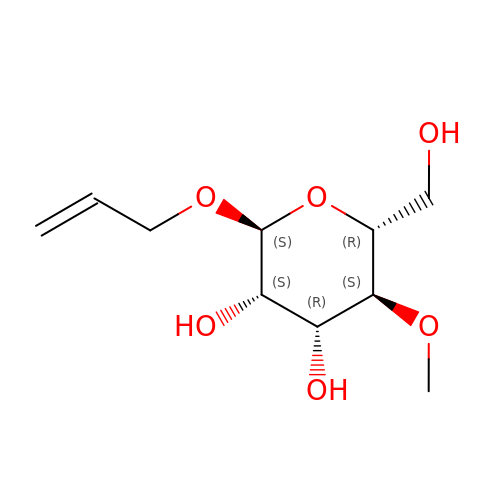prop-2-en-1-yl 4-O-methyl-alpha-D-mannopyranoside | C10 H18 O6 | VOIKDSWIMJSKCR-SPFKKGSWSA-N> MATSNLLKNKGSLQFEDKWDFMRPIVLKLLRQESVTKQQWFDLFSDVHAVCLWDDKGPAKIHQALKEDILEFIKQAQARVLSHQDDTALLKAYIVEWRKFFTQCDILPKPFCQLEITLMGKQGSNKKSNVEDSIVRKLMLDTWNESIFSNIKNRLQDSAMKLVHAERLGEAFDSQLVIGVRESYVNLCSNPEDKLQIYRDNFEKAYLDSTERFYRTQAPSYLQQNGVQNYMKYADAKLKEEEKRALRYLETRRECNSVEALMECCVNALVTSFKETILAECQGMIKRNETEKLHLMFSLMDKVPNGIEPMLKDLEEHIISAGLADMVAAAETITTDSEKYVEQLLTLFNRFSKLVKEAFQDDPRFLTARDKAYKAVVNDATIFKLELPLKQKGVGLKTQPESKCPELLANYCDMLLRKTPLSKKLTSEEIEAKLKEVLLVLKYVQNKDVFMRYHKAHLTRRLILDISADSEIEENMVEWLREVGMPADYVNKLARMFQDIKVSEDLNQAFKEMHKNNKLALPADSVNIKILNAGAWSRSSEKVFVSLPTELEDLIPEVEEFYKKNHSGRKLHWHHLMSNGIITFKNEVGQYDLEVTTFQLAVLFAWNQRPREKISFENLKLATELPDAELRRTLWSLVAFPKLKRQVLLYEPQVNSPKDFTEGTLFSVNQEFSLIKNAKVQKRGKINLIGRLQLTTERMREEENEGIVQLRILRTQEAIIQIMKMRKKISNAQLQTELVEILKNMFLPQKKMIKEQIEWLIEHKYIRRDESDINTFIYMA;> MVAASSRLMKELEEIRKAGMKNFRNI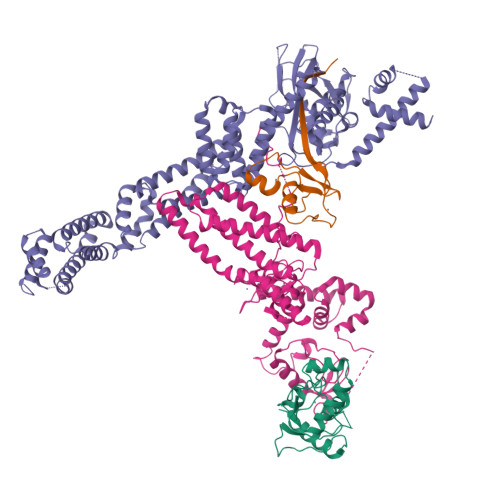QVDEANLLTWQGLIVPDNPPYDKGAFRIEINFPAEYPFKPPKITFKTKIYHPNIDEKGQVCLPVISAENWKPATKTDQVIQSLIALVNDPQPEHPLRADLAEEYSKDRKKFAKNAEEFTKKYGEKRPVD;> MSVDMNSQGSDSNEEDYDPNCEEEEEEEEDDPGDIEDYYVGVASDVEQQGADAFDPEEYQFTCLTYKESEGALNEHMTSLASVLKVSHSVAKLILVNFHWQVSEILDRYKSNSAQLLVEARVQPNPSKHVPTSHPPHHCAVCMQFVRKENLLSLACQHQFCRSCWEQHCSVLVKDGVGVGVSCMAQDCPLRTPEDFVFPLLPNEELREKYRRYLFRDYVESHYQLQLCPGADCPMVIRVQEPRARRVQCNRCNEVFCFKCRQMYHAPTDCATIRKWLTKCADDSETANYISAHTKDCPKCNICIEKNGGCNHMQCSKCKHDFCWMCLGDWKTHGSEYYECSRYKENPDIVNQSQQAQAREALKKYLFYFERWENHNKSLQLEAQTYQRIHEKIQERVMNNLGTWIDWQYLQNAAKLLAKCRYTLQYTYPYAYYMESGPRKKLFEYQQAQLEAEIENLSWKVERADSYDRGDLENQMHIAEQRRRTLLKDFHDT;> MADVEDGEETCALASHSGSSGSKSGGDKMFSLKKWNAVAMWSWDVECDTCAICRVQVMDACLRCQAENKQEDCVVVWGECNHSFHNCCMSLWVKQNNRCPLCQQDWVVQRIGK2-(2-(3,4-DICHLOROPHENYL)-5-(ISOPROPYLAMINO)-6-OXOPYRIMIDIN-1(6H)-YL)-N-((S)-1-OXO-1-(THIAZOL-2-YL)-5-GUANIDINOPENTAN-2-YL)ACETAMIDE 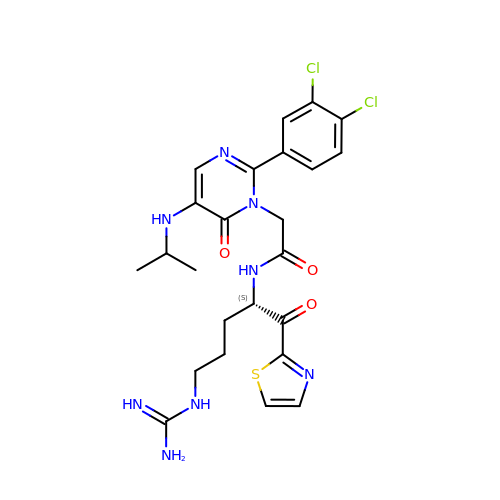| C24 H28 Cl2 N8 O3 S | LJLKTQRJOBRXIB-KRWDZBQOSA-N>SGSMAAGERWWRFRVDYHAGPMDDLILDGVRPAFAAFAAQAPMAYFLRHWRRGPHLRIYVSTTREALEAVVRPAIEHVVGGYLRARPSPGMADPSAFLPLHERLAELEGEDGPLMPWSPDNTIHAEGERPEPLTVRDVLLADFYADTTPSVYHALERVRSGASLPTIAFDLVVATAHALSTGGLPVARTSLRSHAEAYLARRSDGVRLRELWRDHYARNREAFTERLIAVASSAESAENGAHLPHVREWVRRLRPIRERARALLESGELTLEYASPAEGARDLPSLAEVSAFHRELESRPEWARLRDSPAFGAYRLVINCTYLHLTRLGLTPHQ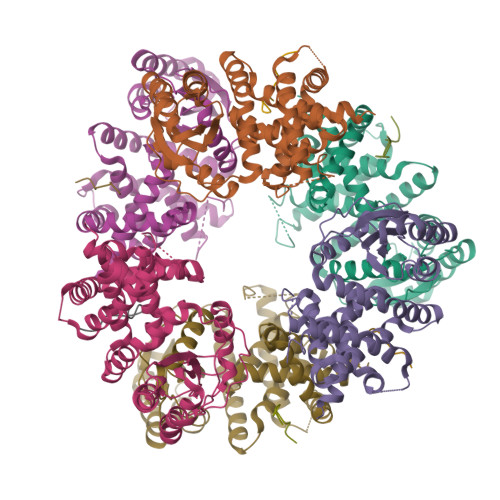RFLVCHLAADAAADVYGIAAHEEVATR[6x];>[6x]MDLNDLPMDVFELADS> MYYSLMRESKVIVEYDGRAFHFDALSNYDVQTSYEEFKTLRRTIHRRTNYADSVINAQTPSSISLAINFSNTLTEANFFEWLGFDRKGNTFLLPLYSNNI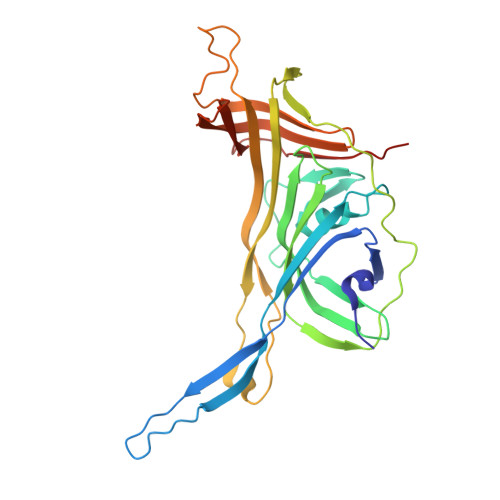EPIMFNIYIVNKDNNCVYFENCYVSTVDFSLDKNIPILNVGIESGKFSEVSTYREAASIIQGEAMSYSPVIVSTNGNILPGLISASLSFQQQCSWREDKSVFDINKIYNNKRAYVNEMNASATISLYYLKRFAGDMVYNIEPETDVPLNIRNNNISIDFPLARISKRLNFSDVYKVEWDIIPTASSDPVRIDFFGEIKND(8S)-N~2~-[(4-tert-butylphenyl)methyl]-N~7~,N~7~-dimethyl-5-[(morpholin-4-yl)methyl][1,2,4]triazolo[1,5-a]pyrimidine-2,7-diamine 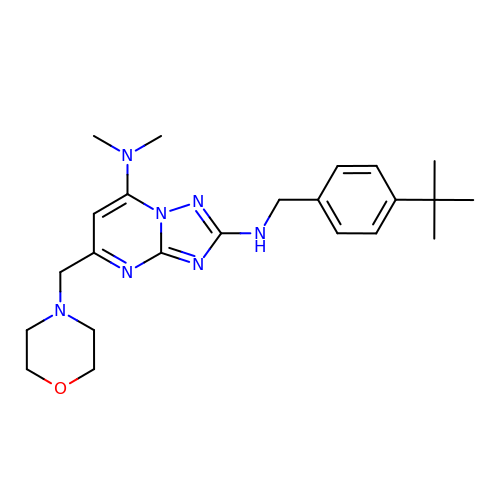| C23 H33 N7 O | RFOXHOSYULBELK-UHFFFAOYSA-N> NNVGPIIRGDLVVEPVIETAEIDNPGKEITV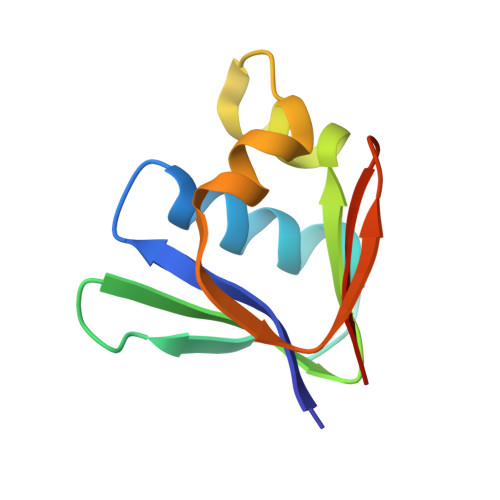EDRRAYVRIAAEGELILTRKTLEEQLGRPFNMQELEINLASFAGQIQADEDQIRFYFDKTM> TFSYTLEDHTKQAFGIMNELRLSQQLCDVTLQVKYQDAPAAQFMAHKVVLASSSPVFKAMFTNGLREQGMEVVSIEGIHPKVMERLIEFAYTASISMGEKCVLHVMNGAVMYQIDSVVRACSDFLVQQLDPSNAIGIANFAEQIGCVELHQRAR;> DEKYVNSIWDLLKNAIQEIQRKNNSGLSFEELYRNAYTMVLHKHGEKLYTGLREVVTEHLINKVREDVLNSLNNNFLQTLNQAWNDHQTAMVMIRDILMYMDRVYVQQNNVENVYNLGLIIFRDQVVRYGCIRDHLRQTLLDMIARERKGEVVDRGAIRNACQMLMILGLEGRSVYEEDFEAPFLEMSAEFFQMESQKFLAENSASVYIKKVEARINEEIERVMHCLDKSTEEPIVKVVERELISKHMKTIVEMENSGLVHMLKNGKTEDLGCMYKLFSRVPNGLKTMCECMSSYLREQGKALVSEEGEGKNPVDYRQGLDDLKSRFDRFLLESFNNDRLFKQTIAGDFEYFLNLN

KEAP1 promotes the ubiquitin-dependent degradation of NRF2 by assembling into a CUL3-dependent ubiquitin ligase complex. Oxidative and electrophilic stress inhibit KEAP1 allowing NRF2 to accumulate for the transactivation of stress response genes.

To date there are no structures of the KEAP1-CUL3 interaction nor binding data to show the contributions of different domains to their binding affinity. We determined a crystal structure of the BTB and 3-box domains of human KEAP1 in complex with the CUL3 N-terminal domain that showed a heterotetrameric assembly with 2:2 stoichiometry. To support the structural data, we developed a versatile TR-FRET-based assay system to profile the binding of BTB-domain-containing proteins to CUL3 and determine the contribution of distinct protein features, revealing the importance of the CUL3 N-terminal extension for high affinity binding. We further provide direct evidence that the investigational drug CDDO does not disrupt the KEAP1-CUL3 interaction, even at high concentrations, but reduces the affinity of KEAP1-CUL3 binding.>GPMGTDWPVYHRIDGPIVMIGFGSIGRGTLPLIERHFAFDRSKLVVIDPSDEARKLAEARGVRFIQQAVTRDNYRELLVPLLTAGPGQGFCVNLSVDTSSLDIMELARENGALYIDTVVEPWLGFYFDPDLKPEARSNYALRETVLAARRNKPGGTTAVSCCGANPGMVSWFVKQALVNLAADLGVTGEEPTTREEWARLAMDLGVKGIHIAERDTQRASFPKPFDVFVNTESVEGFVSEGLQPAELGWGTFERWMPDNARGHDSGCGAGIYLLQPGANTRVRSWTPTAMAQYGFLVTHNESISIADFLTVRDAAGQAVYRPTCHYAYHPCNDAVLSLHEMFGSGKRQSDWRILDETEIVDGIDELGVLLYGHGKNAYWYGSQLSIEETRRIAPDQNATGLQVSSAVLAGMVWALENPNAGIVEADDLDFRRCLEVQTPYLGPVVGVYTDWTPLAGRPGLFPEDIDTSDPWQFRNVLVRD[2x]

Bacterial HSS is mostly found in α-proteobacteria and in some β- and γ-proteobacteria, including pathogenic strains such as Legionella pneumophila, Brucella spp. and various P. aeruginosa strains, including PA7 and PA14. It catalyzes the conversion of two molecules of putrescine (PUT; 1,4-diaminobutane) into one molecule of sym-homospermidine [HSP; bis(4-aminobutyl)amine] as the main reaction along with several side reactions (Ober et al., 1996; Böttcher et al., 1994). Bacterial HSS is NAD+-dependent, active at neutral to basic pH with an optimum at pH ∼8.8, and shows increased activity in the presence of 50 mM potassium ion. BvHSS forms a dimer, with each subunit containing a boot-shaped substrate-binding pocket between an NAD(P)-binding Rossmann-like domain and an HSS-like domain. The cofactor NAD+ is bound as a prosthetic group in the binding pocket with its nicotinamide ring being part of the active site.

The W229E variant was generated to scrutinize the possible stabilization of positively charged reaction components by a salt bridge instead of a cation–π interaction. The only exception was the structure of the BvHSS variant W229E, which could only be refined to a maximum resolution of 2.76 Å. Apart from the exchanged residues, all residues in the binding pockets of these variants superimpose almost perfectly onto the wild-type residues without considerable deviations. Regarding the structure of the inactive variant W229E, the location of the carboxyl group of Glu229 is probably not completely fixed. The carboxyl group is rotated between the two subunits of the variant and the omit maps reveal a lack of electron density clearly supporting the location of the carboxyl group. A reduced occupancy of the carboxyl group at a defined location due to flexibility of the side chain or radiation damage affecting the carboxyl group should therefore be assumed. In any case, the side chain of Glu229 is able to protrude into the active site, as modeled in the variant structure, which would sterically interfere with substrate binding. In conclusion, the inactivity of both variants W229E and W229K is not necessarily caused by their inability to provide cation–π interaction but might rather result from steric issues or an enlarged space enabling increased flexibility of the substrate. Still, both variants are inactive as expected for a cation–π-dependent reaction mechanism.>[2x]MRGSHHHHHHMSIITDVYAREVLDSRGNPTLEVEVYTESGAFGRGMVPSGASTGEHEAVELRDGDKSRYGGLGTQKAVDNVNNIIAEAIIGYDVRDQQAIDRAMIALDGTPNKGKLGANAILGVSIAVARAAADYLEIPLYSYLGGFNTKVLPTPMMNIINGGSHSDAPIAFQEFMILPVGAPTFKEALRYGAEIFHALKKILKSRGLETAVGDEGGFAPRFEGTEDGVETILAAIEAAGYVPGKDVF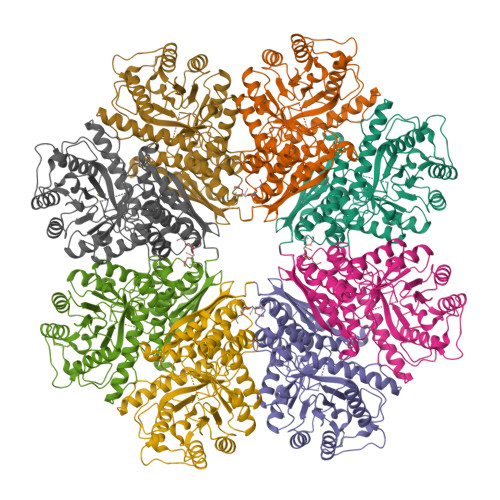LGFDCASSEFYDKERKVYDYTKFEGEGAAVRTSAEQIDYLEELVNKYPIITIEDGMDENDWDGWKALTERLGKKVQLVGDDFFVTNTDYLARGIQEGAANSILIKVNQIGTLTETFEAIEMAKEAGYTAVVSHRSGETEDSTIADIAVATNAGQIKTGSLSRTDRIAKYNQLLRIEDQLGEVAEYRGLKSFYNLKK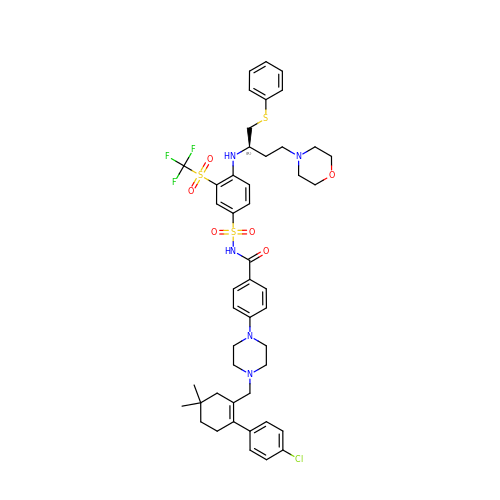4-(4-{[2-(4-chlorophenyl)-5,5-dimethylcyclohex-1-en-1-yl]methyl}piperazin-1-yl)-N-[(4-{[(2R)-4-(morpholin-4-yl)-1-(phenylsulfanyl)butan-2-yl]amino}-3-[(trifluoromethyl)sulfonyl]phenyl)sulfonyl]benzamide | C47 H55 Cl F3 N5 O6 S3 | JLYAXFNOILIKPP-KXQOOQHDSA-N>AYTTFSATKNDQLKEPMFFGQP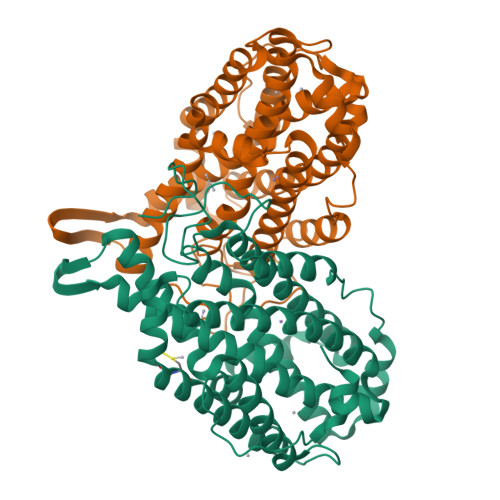VQVARYDQQKYDIFEKLIEKQLSFFWRPEEVDVSRDRIDYQALPEHEKHIFISNLKYQTLLDSIQGRSPNVALLPLISIPELETWVETWAFSETIHSRSYTHIIRNIVNDPSVVFDDIVTNEQIQKRAEGISSYYDELIEMTSYWHLLGEGTHTVNGKTVTVSLRELKKKLYLCLMSVNALEAIRFYVSFACSFAFAERELMEGNAKIIRLIARDEALHLTGTQHMLNLLRSGADDPEMAEIAEECKQECYDLFVQAAQQEKDWADYLFRDGSMIGLNKDILCQYVEYITNIRMQAVGLDLPFNTRSNPIPWINTWLVSDNVQVAPQEVEVSSYLVGQIDSEVDTDDLSNFQL[2x]(E)-N~2~-({3-hydroxy-2-methyl-5-[(phosphonooxy)methyl]pyridin-4-yl}methylidene)-L-arginine 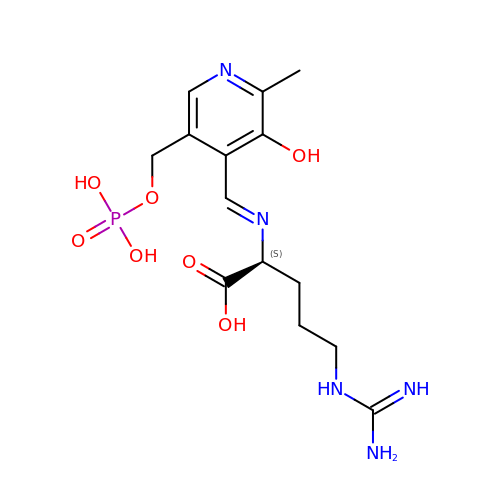| C14 H22 N5 O7 P | PFHOMURYEGODJI-GBCOYWTISA-N> RWRPKKSYKKRTMGLPSTKA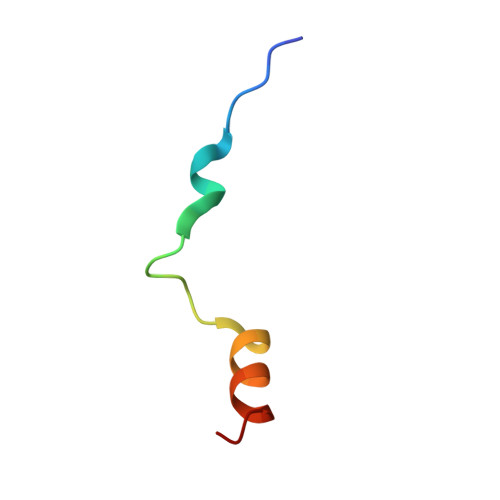RRRWAQMRRG> MVATTSSGGSSVGWPSRLSGVRLHLVTGKGGTGKSTIAAALALTLAAGGRKVLLVEVEGRQGIAQLFDVPPLPYQELKIATAERGGQVNALAIDIEAAFLEYLDMFYNLGIAGRAMRRIGAVEFATTIAPGLRDVLLTGKIKETVVRLDKNKLPVYDAIVVDAPPTGR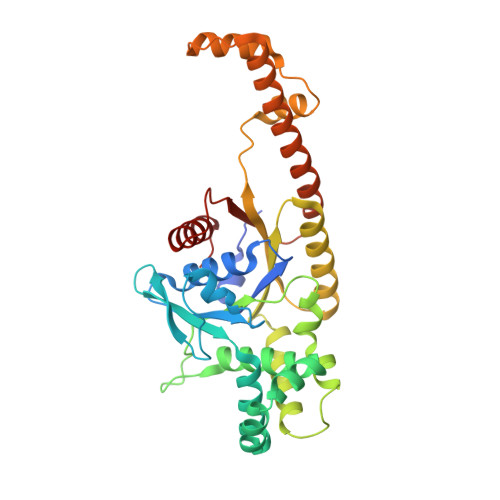IARFLDVTKAVSDLAKGGPVHAQSEGVVKLLHSNQTAIHLVTLLEALPVQETLEAIEELAQMELPIGSVIVNRNIPAHLEPQDLAKAAEGEVDADSVRAGLLTAGVKLPDADFAGLLTETIQHATRITARAEIAQQLDALQVPRLELPTVSDGVDLGSLYELSESLAQQGVR>MKFKWDEFFVTGDPLILGAQVSIALSTIAIIFVLTYFKKWKWLWSEWITTVDHKKLGIMYIISAVIMLFRGGVDGLMMRAQLALPNNSFLDSNHYNEIFTTHGTIMIIFMAMPFLIGLINVVVPLQIGARDVAFPYLNNLSFWTFFVGAMLFNISFVIGGSPNAGWTSYMPLASNDMSPGPGENYYLLGLQIAGIGTLMTGINFMVTILKMRTKGMTLMRMPMFTWTTLITMVIIVFAFPVLTVALALLSFDRLFGAHFFTLEAGGMPMLWANLFWIWGHPEVYIVILPAFGIFSEIISSFARKQLFGYKAMVGSIIAISVLSFLVWTHHFFTMGNSASVNSFFSITTMAISIPTGVKIFNWLFTMYKGRISFTTPMLWALAFIPNFVIGGVTGVMLAMAAADYQYHNTYFLVSHFHYVLIAGTVFACFAGFIFWYPKMFGHKLNERIGKWFFWIFMIGFNICFFPQYFLGLQGMPRRIYTYGPNDGWTTLNFISTVGAFMMGVGFLILCYNIYYSFRYSTREISGDSWGVGRTLDWATSSAIPPHYNFAVLPEVKSQDAFLHMKEEKTELYPESKFKKIHMPSNSGRPFFMSVAFGLAGFGLVFEWYWMGVVGLIGVLLCMVLRSFEYDNGYYISVDEIKETERKISEHHHHHH[2x];>CSNASVLDPKGPVAEQQSDLILLSIGFMLFIVGVVFVLFTIILVKYRDRKGKDNGSYNPEIHGNTFLEVVWTVIPILIVIALSVPTVQTIYSLEKAPEATKDKEPLVVYATSVDWKWVFSYPEQDIETVNYLNIPVDRPILFKISSADSMASLWIPQLGGQKYAMAGMLMDQYLQADKVGTYEGRNANFTGEHFADQEFDVNAVTEKDFNSWVKKTQNEAPKLTKEKYDELMLPENVDELTFSSTHLKYVDHGQDAEYAMEARKRLGYQAVSPHSKTDPFENVKKNEFKKSDDTEE[2x];>[2x]MEHAEHGNSNA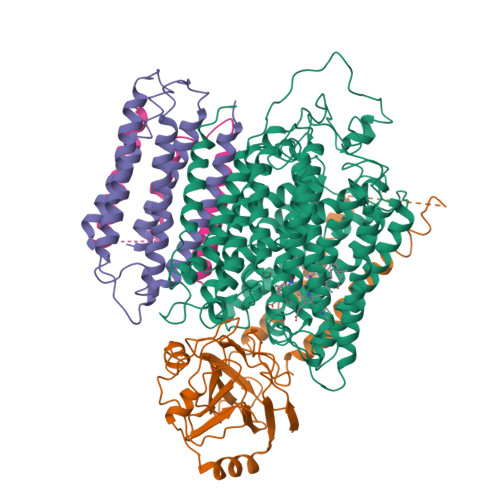PMEYQSETGRLNILGFWIFLGAEIVLFSTLFATFFVLKNRTAGGVLPDELFEVNLVMIMTFLLLISSFTCGIAVHEMRRGSLKGVVIWTIITLLLGAGFVGCEINEFVHYVHEGAALSTSAFWSGFFVLLGTHGTHVTIGIFWITGILIQLKKRGLTPQTSSKIFISSLYWHFLDVVWIFIFTGVYLMGLGGL>GSHMITVATAECFTHANIGLTIHKAAAGYEDFEFKYLFSEEDLKLMKNVRVIS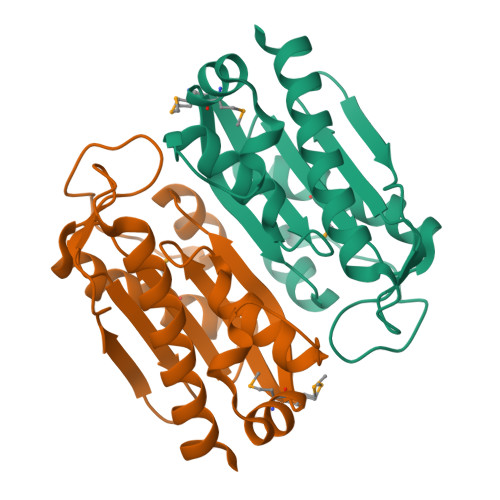AMFVPSIIGVEKLLDIKLPEPDFNYKYAKAYSEEKDLEVAKLMAEGLKKKLNVNISIGSTAGVGRGAICILTDNNRYLFTSDVYANLITFENIKERQKNGIEKGIKRFLEILKKEYF[2x]> IESIIKTATDTVKSEINAELGVVPSLNAVETGATSNTEPEEAIQ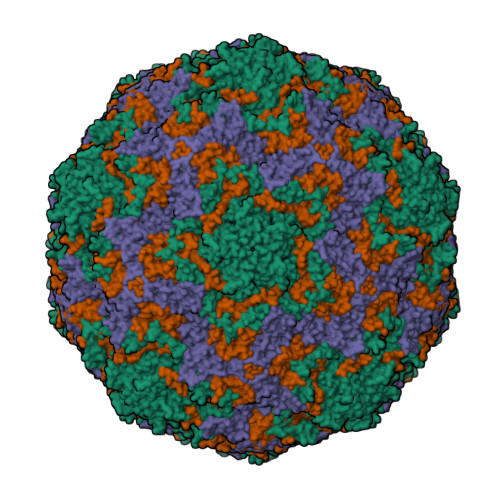TRTVINQHGVSETLVENFLSRAALVSKRSFEYKDHTSSAAQTDKNFFKWTINTRSFVQLRRKLELFTYLRFDAEITILTTVAVNGSSNNTYMGLPNLTLQAMFVPTGALTPEKQDSFHWQSGSNASVFFKISDPPARMTIPFMCINSAYSVFYDGFAGFEKSGLYGINPADTIGNLCVRIVNEHQPVGFTVTVRVYMKPKHIKAWAPRPPRTLPYMSIANANYKGKKRAPNALNAIIGNRDSVKTMPHNIVTT;> GVPTYLLPGSGQFLTTDDHSSAPVLPCFNPTPEMHIPGQVRNMLEVVQVESMMEINNTESAVGMERLKVDISALTDVDQLLFNIPLDIQLDGPLRNTLVGNISRYYTHWSGSLEMTFMFCGSFMATGKLILCYTPPGGSCPTTRETAMLGTHIVWDFGLQSSVTLIIPWISGSHYRMFNNDAKSTNANVGYVTCFMQTNLIVPSESSDTCSLIGFIAAKDDFSLRLMRDSPDIGQIDHLHAAEAAYQ;> SPSAEACGYSDRVLQLKLGNSAIVTQEAANYCCAYGEWPNYLPDHEAVAIDKPTQPETATDRFYTLKSVKWEAGSTGWWWKLPDALNNIGMFGQNVQHHYLYRSGFLIHVQCNATRFHQGALLVVAIPEHQRGAHNTNTSPGFDDIMKGEEGGTFNHPYVLDDGTSLACATIFPHQWINLRTNNSATIVLPWMNAAPMDFPLRHNQWTLAIIPVVPLGTRTMSSMVPITVSIAPMCCEFNGLRHAITQ;> GAQVTRQQTGTHENANIATNGSHITYNQINFYKDSYAASASKQDFSQDPSKFTEPVVEGLKAGAPVLK>MGSVGRVTAPEPLSAFHQVAEFVSGEAVLDDWLKQKGLKNQALGAARTFVVCKKDTKQVAGFYSLATGSVNHTEATGNLRRNMPDPIPVIILARLAVDLSFHGKGLGADLLHDAVLRCYRVAENIGVRAIMVHALTEEAKNFFIHHGFKSSQTQQRTLFLRLPQ[6x];>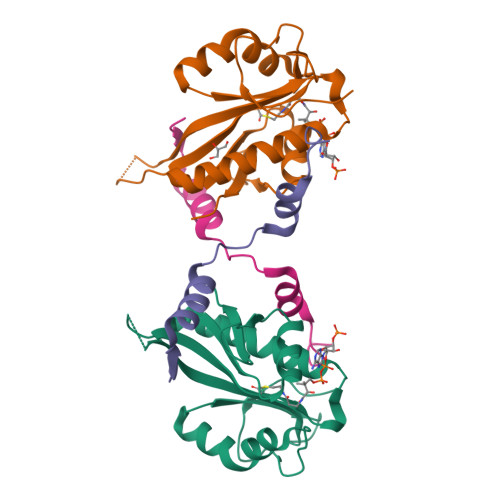[6x]GSFNFNDEQYEEFINLLDAPVADDPVIEKLLARKPQWDV>MADEIAKAQVARPGGDTIFGK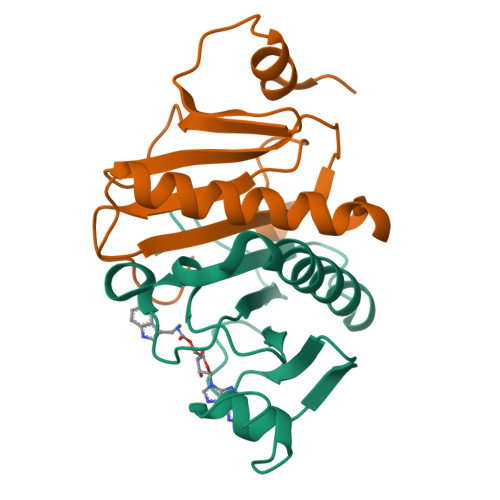IIRKEIPAKIIFEDDRCLAFHDISPQAPTHFLVIPKKHISQISVAEDDDESLLGHLMIVGKKCAADLGLNKGYRMVVNEGSDGGQSVYHVHLHVLGGRQMHWPPG[2x]>[2x]PL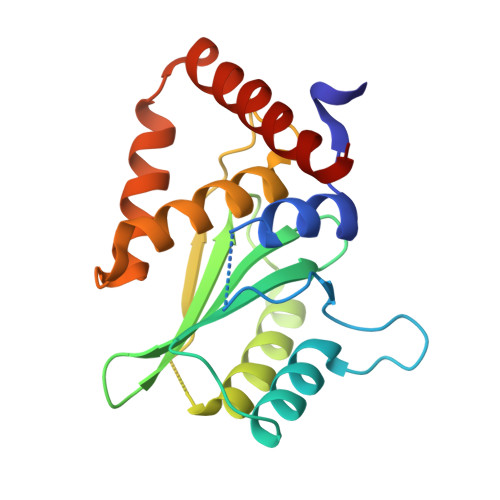GSRMLSSDELAAATQGLVQESPLLSVNYPIGLIHPTTKENILSTQLLEKIAQSGLSHNEVFLVNTGDHWLLCLFYKLAEKIKCLIFNTYYDLNENTKQEIIEAAKIAGISESDEVNFIEMNLQNNVPNGCGLFCYHTIQLLSNAGQNDPATTLREFAENFLTLSVEEQALFNTQTRRQIYEYSLQ>GGTTGGTGTGGTTGG[6x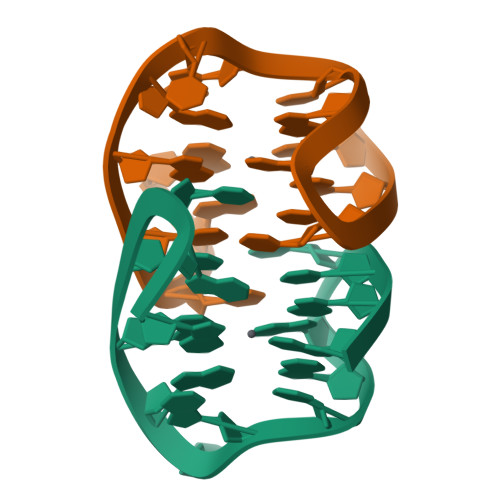]>[4x]MAEKNYVMAIDQGTTSSRAIIFDRNGKKIGSSQKEFPQYFPKSGWVEHNANEIWNSVQSVIAGAFIESGIRPEAIAGIGITNQRETTVVWDKTTGQPIANAIVWQSRQSSPIADQLKVDGHTEMIHEKTGLVIDAYFSATKVRWLLDNIEGAQEKADNGELLFGTIDSWLVWKLTDGQVHVTDYSNASRTMLYNIHKLEWDQEILDLLNIPSSML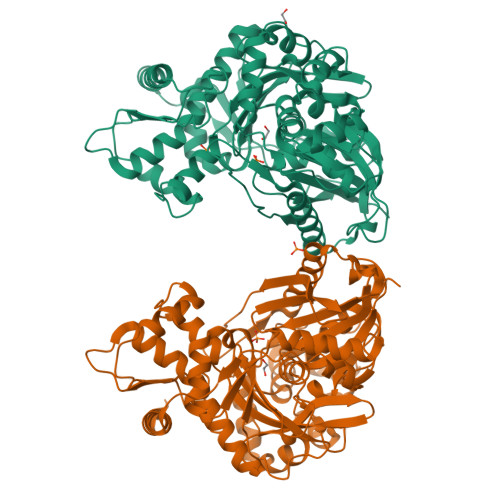PEVKSNSEVYGHTRSYEFYGSEVPIAGMAGDQQAALFGQMAFEKGMIKNTYGTGAFIVMNTGEEPQLSDNDLLTTIGYGINGKVYYALEGSIFVAGSAIQWLRDGLRMIETSPQSEELAAKAKGDNEVYVVPAFTGLGAPYWDSEARGAVFGLTRGTTKEDFVRATLQAVAYQSKDVIDTMKKDSGIDIPLLKVDGGAAKNDLLMQFQADILDIDVQRAANLETTALGAAYLAGLAVGFWKDLDELKSMAEEGQMFTPEMPAEERDNLYEGWKQAVAATQTFKFKAKKEGE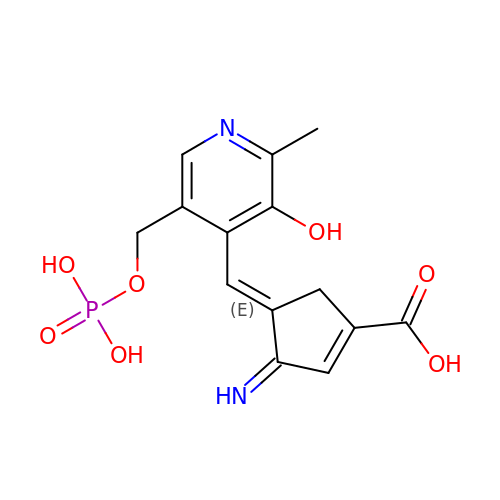(3E,4E)-4-({3-hydroxy-2-methyl-5-[(phosphonooxy)methyl]pyridin-4-yl}methylidene)-3-iminocyclopent-1-ene-1-carboxylic acid | C14 H15 N2 O7 P | NSAJRPMHFRLIPA-LEGHTLSWSA-N>[2x]ASRDPQGRPDSPRERTPKGKPHAQQPGRASASDSSAPWSRSTDGTILAQKLAEEVPMDVASYLYTGDSHQLKRANCSGRYELAGLPGKWPALASAHPSLHRALDTLTHATNFLNVMLQSNKSREQNLQDDLDWYQALVWSLLEGEPSISRAAITFSTDSLSAPAPQVFLQATREESRILLQDLSSSAPHLANATLETEWFHGLRRKWRPHLHRRGPNQGPRGLGHSWRRKDGLGGDKSHFKWSPPYLECENGSYKPGWLVTLSSAIYGLQPNLVPEFRGVMKVDINLQKVDIDQCSSDGWFSGTHKCHLNNSECMPIKGLGFVLGAYECICKAGFYHPGVLPVNNFRRRGPDQHISGSTKDVSEEAYVCLPCREGCPFCADDSPCFVQEDKYLRLAIISFQALCMLLDFVSMLVVYHFRKAKSIRASGLILLETILFGSLLLYFPVVILYFEPSTFRCILLRWARLLGFATVYGTVTLKLHRVLKVFLSRTAQRIPYMTGGRVMRMLAVILLVVFWFLIGWTSSVCQNLEKQISLIGQGKTSDHLIFNMCLIDRWDYMTAVAEFLFLLWGVYLCYAVRTVPSAFHEPRYMAVAVHNELIISAIFHTIRFVLASRLQSDWMLMLYFAHTHLTVTVTIGLLLIPKFSHSSNNPRDDIATEAYEDELDMGRSGSYLNSSINSAWSEHSLD

GPR158, a class C orphan GPCR, functions in cognition, stress-induced mood control, and synaptic development. Among class C GPCRs, GPR158 is unique as it lacks a Venus flytrap-fold ligand-binding domain and terminates Gαi/o protein signaling through the RGS7-Gβ5 heterodimer. Here, we report the cryo-EM structures of GPR158 alone and in complex with one or two RGS7-Gβ5 heterodimers. GPR158 dimerizes through Per-Arnt-Sim-fold extracellular and transmembrane (TM) domains connected by an epidermal growth factor-like linker.

We determined the overall structure of apo GPR158 at an average resolution of 3.5 Å. GPR158 consists of an α/β-fold extracellular domain, a cysteine-rich (CR) domain with an epidermal growth factor (EGF)-like fold, and 7TM domain. GPR158 forms an elongated shape (79 × 147 × 49 Å3) and dimerizes through both extracellular and TM domains. The extracellular domain dimerizes through the side-by-side packing of α4 and α5′ and α5 and α4′ helices (′ indicates the second protomer) in a parallel manner, with a buried surface area of 1806 Å2. The most notable feature of a TM domain is extensive ionic networks present in three layers. Layer III contains an ionic lock, a hallmark of the inactive state in other GPCRs, by tethering TM3, TM6, and ICL3. Overall, the extensive ionic and polar networks in the three layers stabilize TM3, TM5, TM6, TM7, ICL1, and ICL3 in apo GPR158. As a result, the space inside the GPR158 TM domain is not sufficient for the ligand binding. In apo GPR158, the TM4/5 helices are arranged in an inverted V-shape at the dimeric interface. The GPR158 TM domain exhibits both inactive and active features of class C GPCRs; hence, we cannot elucidate whether apo GPR158 is in an inactive, partially active or fully active state that can directly couple to the Gαβγ heterotrimer.Zinc is essential for virulence and survival and is acquired solely by the ABC transporter, AdcCB, and two Zn2+-specific cluster A-I SBPs, AdcA and AdcAII, in S. pneumoniae. Although both SBPs share this structural core, AdcA also has a C-terminal domain (residues 322 to 501; here termed AdcAC) that is structurally related to ZinT, a periplasmic protein from E. coli and Salmonella. The AdcAC domain is linked to the N-terminal cluster A-I domain of AdcA (residues 1 to 311, henceforth referred to as AdcAN) by an 11-amino-acid linking region. Collectively, our data show that the AdcAN domain is necessary and sufficient for Zn2+ acquisition, with the AdcAC domain and the His-rich loop aiding in Zn2+ recruitment during growth under Zn2+-restricted conditions.

The AdcAC domain has a lipocalin-like fold of an 8-stranded up-and-down β-barrel (β9-16) and a helical region of four short helices (α11 to α15). The structure of the AdcAC domain was further analyzed compared to a truncated AdcA variant lacking AdcAN, AdcAC (residues 326 to 501). The structure of metal-free truncated AdcAC was also determined, showing that only minor conformational changes are induced by metal binding. The metal-binding site in the AdcAC domain is also tightly defined. However, it is highly solvent accessible and is permissive for interaction with Co2+ and Ni2+ ions, similar to ZinT homologs.

> DTKTVQNGYFEDAAVKDRTLSDYAGNWQSVYPFLEDGTFDQVFDYKAKLTGKMTQAEYKAYYTKGYQTDVTKINITDNTMEFVQGGQSKKYTYKYVGKKILTYKKGNRGVRFLFEATDADAGQFKYVQFSDHNIAPVKAEHFHIFFGGTSQETLFEEMDNWPTYYPDNLSGQEIAQEMLAH7-[3-(aminomethyl)-4-propoxyphenyl]-4-methylquinolin-2-amine | C20 H23 N3 O | 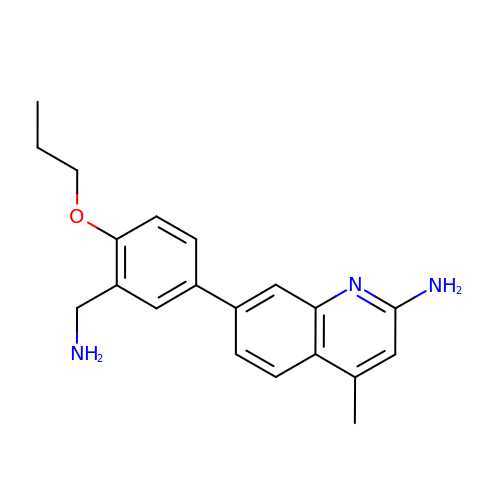WKYWHPWEQYJUAT-UHFFFAOYSA-N>[4x]MAAVSGKSEAAEIEAGDRLDALRDQLQRYETPIIQTILARS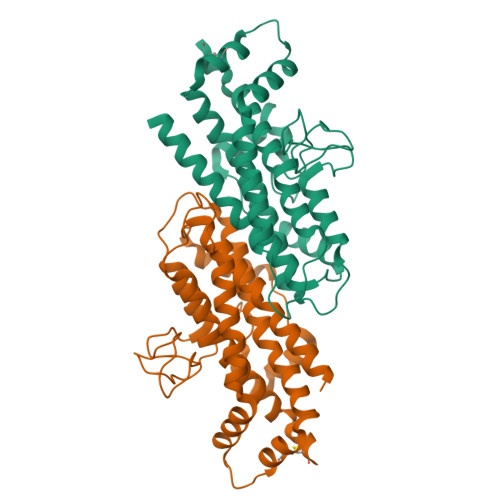ALGGRAPSEQDEVRAALSRNAFEPSEVISEWLQTESGARFRSTRPLPPAVEFITPVVLSRDTVLDKPVVGKGIFPIGRRPQDPTNMDEFLDTSLLSLNQSSTVDLASAVSLDVSLLHLVSARVLLGYPIALAKFDWLHDNFCHILTNTTLSKSQKLANIIQQLTDHKQEVNVLSRVEQKSKSLSHLFRNDIPYPPHTQDRILRLFQAYLIPITTQIEAAAILDHANKCTLEHHHHHH>METLFSGIQPSGIPTIGNYIGALKQFVDVQNDYDCYFCIVDQHAITMPQDRLKLRKQTRQLAAIYLASGIDPDKATLFIQSEVPAHVQAGWMLTTIASVGELERMTQYKDKAQKAVEGIPAGLLTYPPLMAADIVLYNTNIVPVGDDQKQHIELTRNLVDRFNSRYNDVLVKPEIRMPKVGGRVMSLQDPTRKMSK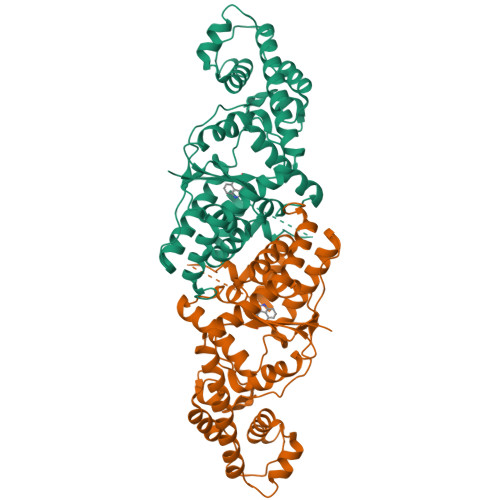SDDNAKNFISLLDEPNVAAKKIKSAVTDSDGIIKFDRDNKPGITNLISIYAGLTDMPIKDIEAKYEGEGYGKFKGDLAEIVKAFLVEFQEKYESFYNSDKLDDILDQGRDKAHKVSFKTVKKMEKAMGLGRKRHHHHHH[3x]> MSLVLMAQATKPEQLQQLQTTYPDWTFKDAAAVTAADYDQIEVMYGNHPLLKTILARPTNQLKFVQVISAGVDYLPLKALQAAGVV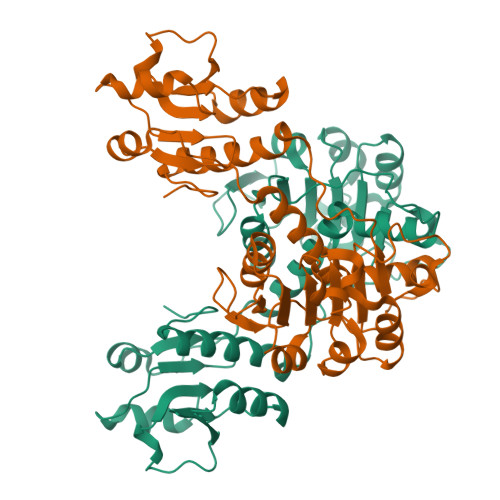VANTSGIHADAISESVLAAMLSVVRGYHAAWLNQRGARQWALPMTTSTLTGQQLLIYGTGQIGQSLAAKASALGMHVIGVNTTGHPADHFHETVAFTATADALATANFIVNALPLTPTTHHLFSTELFQQTKQQPMLINIGRGPAVDTTALMTALDHHQLSMAALDVTEPEPLPTDHPLWQRDDVLITPHISGQIAHFRATVFPIFAANFAQFVKDGTLVRNQVDLNRGYEGHHHHHH>[2x]GMKVPEAAISRLITYLRILEELEAQGVHRTSSEQLGELAQVTAFQVRKDLSYFGSYGTRGVGYTVPVLK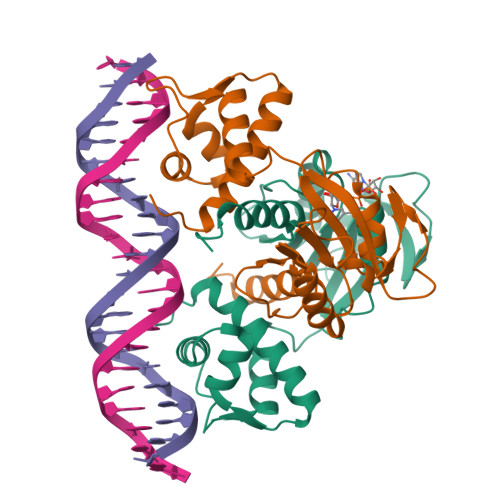RELRHILGLNRKWGLCIVGMGRLGSALADYPGFGESFELRGFFDVDPEKVGRPVRGGVIEHVDLLPQRVPGRIEIALLTVPREAAQKAADLLVAAGIKGILNFAPVVLEVPKEVAVENVDFLAGLTRLSFAILNPKWR> IVGGKVCPKGECPWQVLLLVNGAQLCGGTLINTIWVVSAAHCFDKIKNWRNLIAVLGEHDLSEHDGDEQSRRVAQVIIPSTYVPGTTNHDIALLRLHQPVVLTDHVVPLCLPERTFSERTLAFVRFSLVSGWGQLLDRGATALELMVLNVPRLMTQDCLQQSRKVGDSPNITEYMFCAGYSDGSKDSCKGDSGGPHATHYRGTWYLTGIVSWGQGCATVGHFGVYTRVSQYIEWLQK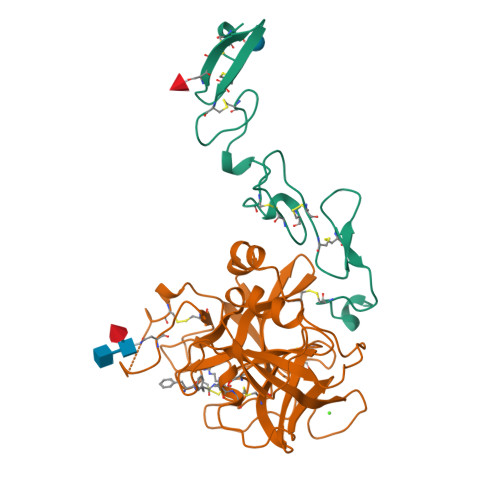LMRSEPRPGVLLRAPFP;> QCASSPCQNGGSCKDQLQSYICFCLPAFEGRNCETHKDDQLICVNENGGCEQYCSDHTGTKRSCRCHEGYSLLADGVSCTPTVEYPCGKIPILEKRNASKPQGR In domain swapping, a protein molecule exchanges its secondary or tertiary structural unit with the corresponding unit of another molecule of the same protein. Cytochrome c (cyt c) is an electron transfer protein existing in the inner membrane space of mitochondria. A hexacoordinated heme is attached covalently to two Cys residues through their sulfur atoms in cyt c. His and Met residues are coordinated to the heme iron of cyt c in its native state.

551 molecules exhibited domain-swapped structures, where the N-terminal Glu1–Met22 (helix 1 and loop 1) and the heme were relocated from the original position observed in the monomer. The hinge loop was constructed with only three amino acids; Thr20, Lys21, and Met22. Interestingly, the active site structure of the dimer was formed by the same amino acids as that of the monomer, but the heme axial ligands (His and Met) belonged to different protomers. We have calculated the root-mean-square deviation (rmsd) for the Cα atoms of the regions from the N-terminus to Asp19 and from Val23 to the C-terminus between the structures of the monomer and each protomer (protomer 1 and protomer 2) of the dimer. The rmsd values of both regions were less than 0.9 Å. These results indicate that the structures of both regions were similar between the monomer and each protomer of the dimer. In addition to these hydrogen bonds, a new hydrogen bond between loop 1 and helix 2 (Asp19AOδ/Lys28BNζ) stabilized the dimer. In the C-terminal region at loop 3, four intramolecular hydrogen bonds seen in the monomer (Ile48CO/Asn64Nδ, Lys49CO/Asn64NH, Ser52CO/Met61NH, and Ser52NH/ Met61CO) were conserved in the dimer. The Fe–His16 and Fe–Met61 bond distances were also similar between the monomer and dimer. Although the redox potential of the dimer decreased by about 30 mV compared to that of the monomer, the dimer exhibited a relatively high redox potential, which is characteristic for cyt c family proteins.

>[2x]EDPEVLFKNKGCVACHAIDTKMVGPAYKDVAAKFAGQAGAEAELAQRIKNGSQGVWGPIPMPPNAVSDDEAQTLAKWVLSQK> SVLFPCKYASSGCEITLPHTEKADHEELCEFRPYSCPCPGASCKWQGSLDAVMPHLMHQHKSITTLQGEDIVFLATDINLPGAVDWVMMQSCFGFHFMLVLEKQEKYDGHQQFFAIVQLIGTRKQAENFAYRLELNGHRRRLTWEATPRSIHEGIAT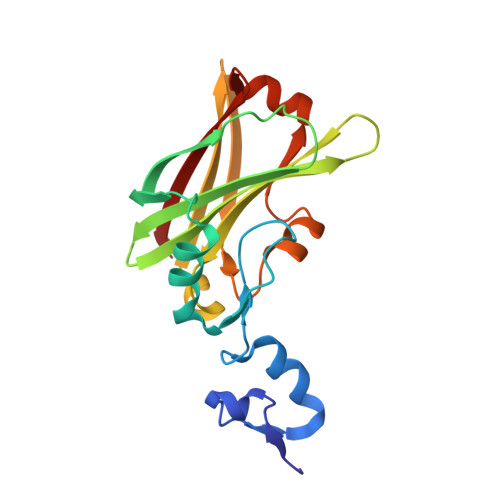AIMNSDCLVFDTSIAQLFAENGNLGINVTISMC>GNVDLVFLFDGSMSLQPDEFQKILDFMKDVMKKLSNTSYQFAAVQFSTSYKTEFDFSDYVKWKDPDALLKHVKHMLLLTNTFGAINYVATEVFREELGARPDATKVLIIITDGEATDSGNIDAAKDIIRYIIGIGKHFQTKESQETLHKFASKPASEFVKILDTFEK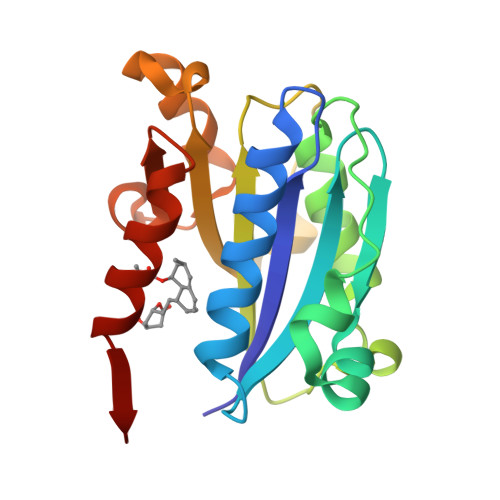LKDLFTELQKKIYVI[2x]2-[(4-{6-[(2,4-difluorophenyl)methoxy]pyridin-2-yl}piperidin-1-yl)methyl]-1-[(1-ethyl-1H-imidazol-5-yl)methyl]-1H-benzimidazole-6-carboxylic acid | C32 H32 F2 N6 O3 | 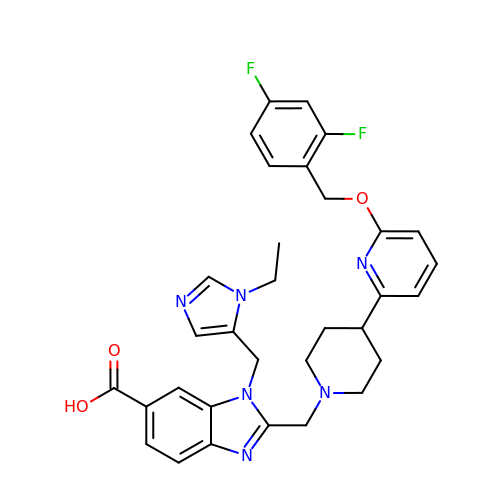IFXPEJAGKQFBER-UHFFFAOYSA-N>[2x]MAAAAAAEVSVDEKLDKLRAEVAKLDQISENEKAGFISLVSRYLSGEAEQI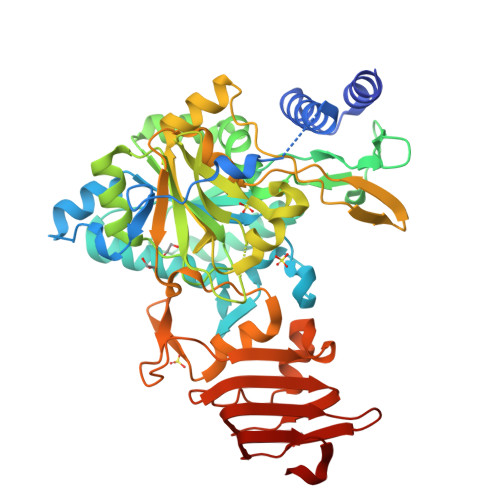EWSKIQTPTDEVVVPYDTLASPPEDLEETKKLLDKLVVLKLNGGLGTTMGCTGPKSVIEVRNGFTFLDLIVIQIESLNKKYGCSVPLLLMNSFNTHDDTQKIVEKYSNSNIEIHTFNQSQYPRIVTEDFLPLPSKGKSGKDGWYPPGHGDVFPSLNNSGKLDILLAQGKEYVFIANSDNLGAIVDIKILNHLINNQNEYCMEVTPKTLADVKGGTLISYEGRVQLLEIAQVPDEHVNEFKSIEKFKIFNTNNLWVNLKAIKRLVEAEALKMEIIPNPKEVDGVKVLQLETAAGAAIRFFDKAIGINVPRSRFLPVKATSDLLLVQSDLYTLVDGFVIRNPARANPANPSIELGPEFKKVANFLARFKSIPSIVELDSLKVSGDVWFGSGITLKGKVTITAKSGVKLEIPDGAVLENKDVNGPEDL>[2x]GGGGGGHMKIIIAGKNDIAVNVTRWLQKKKKNIEIYAICNANDTGIDTFQRSFKKYCKDNLIPIISLAEAYKIDDAIFLSLEFDKIVQPSKFNHNELFNIHFSYLPKYKGMYTSAWPILNGEDTSGVTLHKIDHGIDTGAIIAQKEIIIQPFETAKDLYEKYISEGTSLVIDNISTLLNSEYVEKEQNIKYSSYYSKKTIDYSN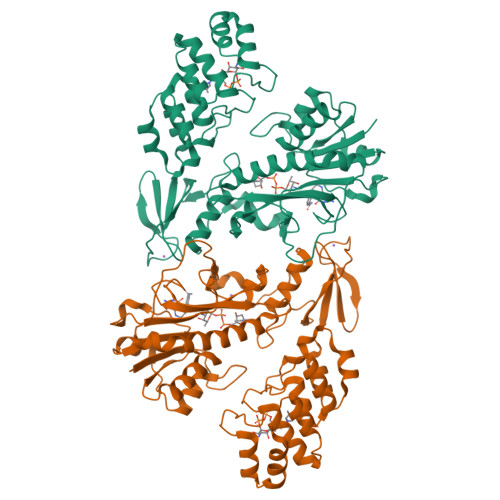LELNFSKTAFEIINQLRAFTFREYQLPKLDGVNIFLGDVLSSRSIMKPGSILERNDKEIIVSTIDYDVVLYKDNFKEILEACKYSDSKYIAKLIRAKSILFEKNIYGWSPVIVAAYHGNIELIKWLVSKGANINDRNYKGTTVAMYFKDYMLKSGDYSGLKMLIDLGLDLTLTDYKDYTVFDYLEKSGNKNLLQYMMAFMK>[2x]MHHHHHHGESIEPLDPSEKANKVLARIFKETELRKLKVLGSGVFGTVHKGVWIPEGESIKIPVCIKVIEDKSGRQSFQAVTDHMLAIGSLDHAHIVRLLGLCPGSSLQLVTQYLPLGSLLDHVRQHRGALGPQLLLNWGVQIAKGMYYLEEHGMVHRNLAARNVLLKSPSQVQVADFGVADLLPPDDKQLLYSEAKTPIKWMA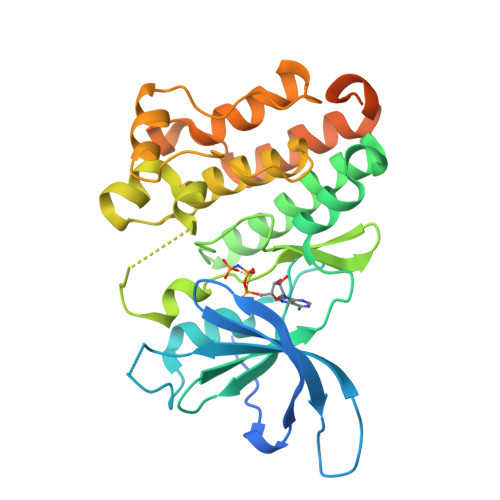LESIHFGKYTHQSDVWSYGVTVWELMTFGAEPYAGLRLAEVPDLLEKGERLAQPQICTIDVYMVMVKCWMIDENIRPTFKELANEFTRMARDPPRYLVIKRESGPGIAPGPEPHGLTNKKLEEVELEPELDLDLDLEAEED> GSASPAVAELCQNTPETFLEASKLLLTYADNILRNPNDEKYRSIRIGNTAFSTRLLPVRGAVECLFEMGFEEGETHLIFPKKASVEQ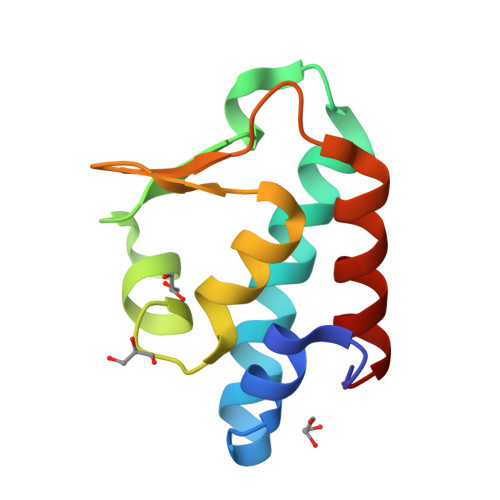LQKIRDLIAIER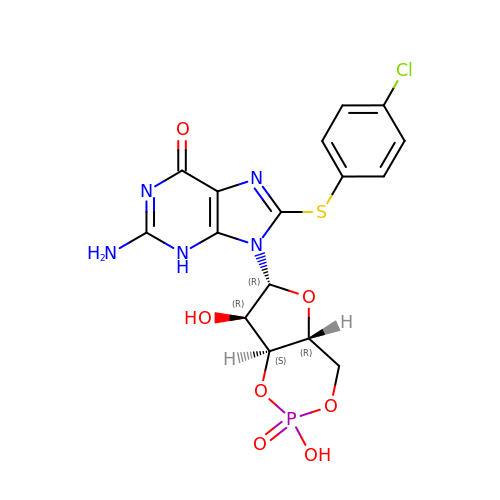2-amino-8-[(4-chlorophenyl)sulfanyl]-9-[(2S,4aR,6R,7R,7aS)-2,7-dihydroxy-2-oxotetrahydro-2H,4H-2lambda~5~-furo[3,2-d][1,3,2]dioxaphosphinin-6-yl]-3,9-dihydro-6H-purin-6-one | C16 H15 Cl N5 O7 P S | ZDJHIEHUVPCEDK-IDTAVKCVSA-N> MLTVLGRLLERNSIYVATIFGGAFAFQGFFDVAVNKWWEEHNKAKLWKNVKGKFLE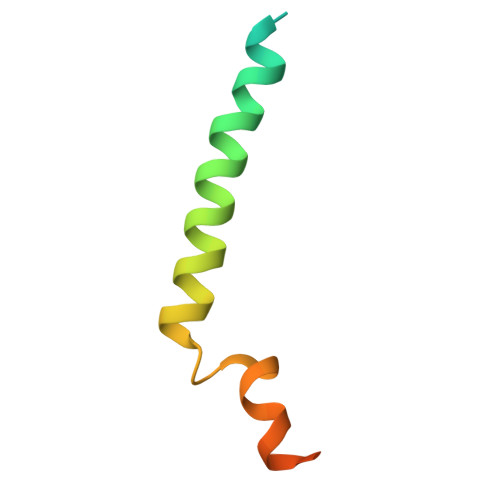GEGEEEDDE> HMDGYYKIKHKASGKFVHPKGGSSNPPNDTNLVLHSDKHERMLFQFVDLGDGYYKIKHKASGKFVHPKGGSSNPPNDTNLVLHSDKHERMLF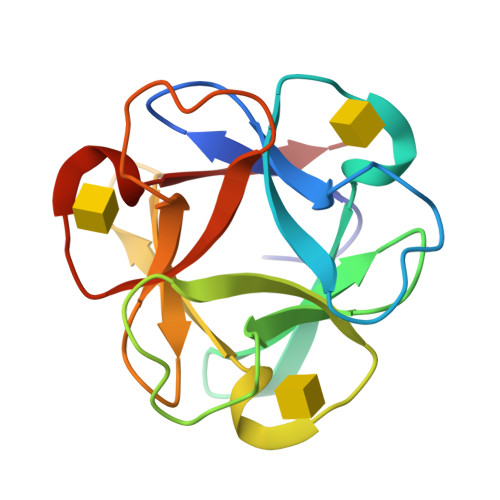QFVDLGDGYYKIKHKASGKFVHPKGGSSNPPNDTNLVLHSDKHERMLFQFVDL>TTGGCGA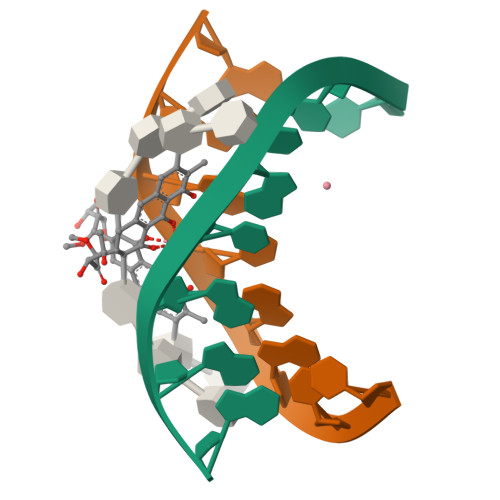A[6x]> ASEALTMIVNLLRS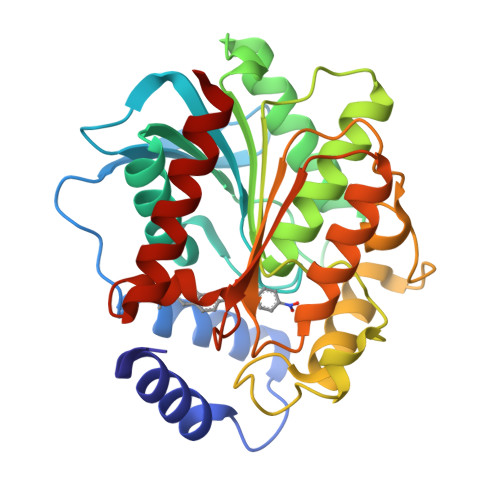QRPLQEPTVEQMRAGLEAMAQMSPLPADVELTTVDAGGVPGAWVRVPESDPDRVVLYLHGGGYVIGSIRTHRDLAQRIARAARCRVLLIDYRLAPEHPHPAAVEDSTRAYRWLLETGSDPKRMAIAGDAAGGGLTVATLVALRDAGVPLPAAAVCLSPWVDLEGIGESMTTKAAVDPMVQREPLLRMASMYLAGQDPRTPLAAPLYADLRGLPPLLIQVGTAETLLDDSVRLAERARAAGVQVTLEPWEDMIHVWQAFAAMLPEGQQAIERIGEFLRQHWQ> MKRMLINATQQEELRVALVDGQRLYDLDIESPGHEQKKANIYKGKITRIEPSLEAAFVDYGAERHGFLPLKEIAREYFPANYSAHGRPNIKDVLREGQEVIVQIDKEERGNKGAALTTFISLAGSYLVLMPNNPRAGGISRRIEGDDRTELKEALASLELPEGMGLIVRTAGVGKSAEALQWDLSFRLKHWEAIKKAAESRPAPFLIHQESNVIVRAFRDYLRQDIGEILIDNPK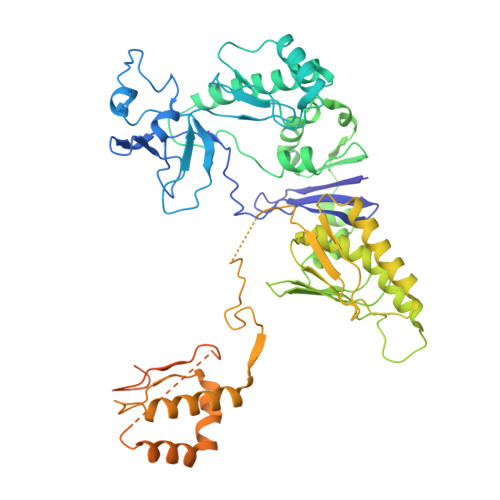VLELARQHIAALGRPDFSSKIKLYTGEIPLFSHYQIESQIESAFQREVRLPSGGSIVIDSTEALTAIDINSARATRGGDIEETAFNTNLEAADEIARQLRLRDLGGLIVICFIDMTPVRHQRAVENRLREAVRQDRARIQISHISRFGLLEMSRQRLSPSLGESSHHVCPRCSGTGTVRDNESLSLSILRLIEEEALKENTQEVHAIVPVPIASYLLNEKRSAVNAIETRQDGVRCVIVPNDQMETPHYHVLRVRKGEETPTLSYMLPKLHEEAMALPSEEEFAERKRPEQPALATFAMPDVPPAPTPAEPAAPVVAPAPKAAPATPAAPAGGEETKPTEQPAPKA> MSSLSRELVFLILQFLDEEKFKETVHKLEQESGFFFNMKYFEEKVHAGEWDEVEKYLSGFTKVDDNRYSMKIFFEIRKQKYLEALDRHDRAKAVDILVKDLKVFSTFNEELYKEITQLLTLENFRENEQLSKYGDTKSARSIMLIELKKLIEAN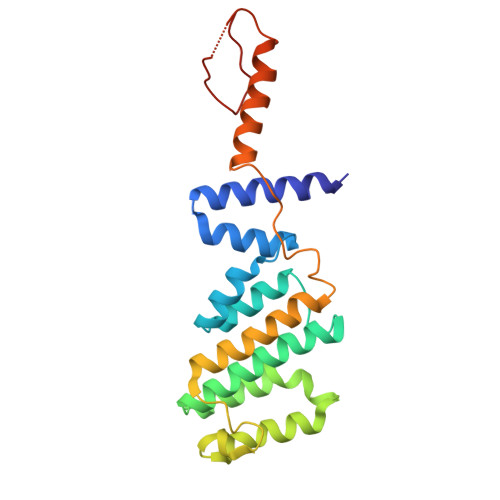PLFREKLVFPTLKASRLRTLINQSLNWQHQLCKNPRPNPDIKTLFTDHTCTPPNG>GITGTWYNQLGSTFIVTAGADGALTGTYESAVGNAESRYVLTGRYDSAPATDGSGTALGWTVAWKNNYRNAHSATTWSGQYVGGAEARINTQWLLTSGTTEANAWKSTLVGHDTFTKVK[4x]

In this work, we use SPA cryo-EM with VPP and Cs-corrector to determine the structure of SA with a molecular weight of ~52 kDa. Different from hemoglobin that consists mostly of α-helices, SA is constituted by mainly β-strands. Our work demonstrates that the VPP can be used in SPA to resolve SA in both the apo-state and biotin-bound state at near-atomic resolution. The atomic model of SA solved previously by X-ray crystallography (PDB 1MEP28) can fit into the EM densities with a correlation coefficient ~0.74, indicating the structural fidelity of SA in its crystallographic and soluble forms.

In the end, we obtained a reconstruction of apo-SA at 3.3 Å resolution (with D2 symmetry applied during the refinement) from a final dataset composed of ~24,000 particles and a reconstruction of the SA–biotin complex at 3.2 Å resolution (with D2 symmetry applied during the refinement) from a final dataset comprising ~45,000 particles. The density of biotin in the SA–biotin reconstruction can be precisely identified with the unambiguous docking of biotin’s atomic model. Compared with the biotin-bound SA, the density corresponding to loop 46–51 in the EM map of apo-SA was missing, indicating that this lid-like loop is flexible without ligand binding. We performed this 3D skip-alignment classification analysis of the apo-SA and biotin-SA datasets separately, and found a rather small occupancy variance around the biotin-binding pocket among the different classes in each dataset, demonstrating unambiguously the lack of biotin in all the monomers of apo-SA and the full occupancy of biotin in all the monomers of biotin-SA. This result occurs because SA has a very strong binding affinity to biotin and the condition of the biotin-SA specimen allowed the full occupancy of the protein’s ligand-binding sites. We also noticed that the orientation distributions of apo-SA and biotin-SA were slightly different. This difference is probably an effect on the surface property of GWI by 4 mM free biotin molecule in the biotin-SA solution. The 39 kDa trimeric dataset had enough signals to generate a correct 3D reconstruction via a global angular search from scratch. Nevertheless, the successful reconstruction of the trimer dataset indicated the capability of solving an asymmetric protein structure with a molecular weight ~39 kDa at near-atomic resolution by SPA cryo-EM.Methylene‐tetrahydropterin reductases catalyze the reduction of a methylene to a methyl group bound to a reduced pterin as C1 carrier in various one‐carbon (C1) metabolisms. F420‐dependent methylene‐tetrahydromethanopterin (methylene‐H4MPT) reductase (Mer) and the flavin‐independent methylene‐tetrahydrofolate (methylene‐H4F) reductase (Mfr) use a ternary complex mechanism for the direct transfer of a hydride from F420H2 and NAD(P)H to the respective methylene group, whereas FAD‐dependent methylene‐H4F reductase (MTHFR) uses FAD as prosthetic group and a ping–pong mechanism to catalyze the reduction of methylene‐H4F. Mutational analysis of four functional amino acids, which are similarly positioned in the three reductase structures, indicated despite the insignificant sequence identity, a common catalytic mechanism with a 5‐iminium cation of methylene‐tetrahydropterin as intermediate protonated by a shared glutamate. Based on mutational and kinetic analysis, evidence has been provided that all three methylene‐tetrahydropterin reductases have the same fold, similar methylene‐tetrahydropterin binding positions, and the same basic catalytic mechanism; however, the binding modes of the C1 carriers and reductants significantly deviate.

Glu6 at the C‐terminal end of β1 points towards the deaza‐isoalloxazine and pterin rings. Position A contains a glutamate residue in all three reductases. In hMfr and jMer, apparent k cat of the equivalent Glu9Gln and Glu6Gln variants decreased from 594 to 1.3 min−1 (0.2%) (Gehl et al., 2023), and from 18,200 to 71 min−1 (0.4%), respectively. Neither variant showed a significant increase in the apparent K m for their respective C1 carrier, suggesting that glutamate and glutamine bind in a related manner. In addition, we obtained the crystal structures of the inactive variants jMer_E6Q, and hMfr_E9Q to exclude perturbations of the active sites. X‐ray structure analysis of the jMer_E6Q and hMfr_E9Q variants were performed and the structures were compared with the wild‐type enzyme, which confirmed unchanged active site architectures compared with the wild‐type enzymes. Based on the mutational analysis at position A, it was possible to extend the proposed model of the catalytic mechanism of MTHFR (Trimmer et al., 2001) not only to Mfr (Gehl et al., 2023) but also to Mer. The mechanism is initiated by the protonation of the C1 carrier to activate this molecule, followed by a hydride transfer from the hydride donor to the activated C1 unit. As the methylene group in methylene‐H4F and methylene‐H4MPT is chemically a rather unreactive aminal, it is unlikely that a hydride can be directly transferred. Therefore, the formation of a positively charged 5‐iminium cation is crucial for catalysis.

> MKFGIQFVPNEPIQKLCYYVKLAEDNGFEYCWITDHYNNRNVYMALTAIAMNTNKIKLGPGVTNPYVRSPAITASAIATLDELSGGRAVLGIGPGDKATFDALGIEWVKPVTTLKESIEVIRKLLAGERVSYEGKVVKIAGAALAVKPIQKAVPVYMGAQGPKMLETAGMIADGVLINASNPKDFEAAIPLIKKGAEAAGRSMDEIDVAAYACMSVDKNADKAKQAAVPVVAFIAAGSPPVVLERHGIDMEKVEAIRNALKSGNFPEAFKNVDDTMLEAFSIYGTPEDVVEKCKKLAEMGVTQIVAGSPIGPNKETAIKLIGKKVIPALKE> MQNSQDFSITELSLPKGGGAITGMGEALTPTGPDGMAALSLPLPISAGRGYAPAFTLNYNSGAGNSPFGLGWDCNVMTIRRRTHFGVPHYDETDTFLGPEGEVLVVADQPRDESTLQGINLGATFTVTGYRSRLESHFSRLEYWQPKTTGKTDFWLIYSPDGQVHLLGKSPQARISNPSQTTQTAQWLLEASVSSRGEQIYYQYRAEDDTGCEADEITHHLQATAQRYLHIVYYGNRTASETLPGLDGSAPSQADWLFYLVFDYGERSNNLKTPPAFSTTGSWLCRQDRFSRYEYGFEIRTRRLCRQVLMYHHLQALDSKITEHNGPTLVSRLILNYDESAIASTLVFVRRVGHEQDGNVVTLPPLELAYQDFSPRHHAHWQPMDVLANFNAIQRWQLVDLKGEGLPGLLYQDKGAWWYRSAQRLGEIGSDAVTWEKMQPLSVIPSLQSNASLVDINGDGQLDWVITGPGLRGYHSQRPDGSWTRFTPLNALPVEYTHPRAQLADLMGAGLSDLVLIGPKSVRLYANTRDGFAKGKDVVQSGDITLPVPGADPRKLVAFSDVLGSGQAHLVEVSATKVTCWPNLGRGRFGQPITLPGFSQPATEFNPAQVYLADLDGSGPTDLIYVHTNRLDIFLNKSGNGFAEPVTLRFPEGLRFDHTCQLQMADVQGLGVASLILSVPHMSPHHWRCDLTNMKPWLLNEMNNNMGVHHTLRYRSSSQFWLDEKAAALTTGQTPVCYLPFPIHTLWQTETEDEISGNKLVTTLRYARGAWDGREREFRGFGYVEQTDSHQLAQGNAPERTPPALTKNWYATGLPVIDNALSTEYWRDDQAFAGFSPRFTTWQDNKDVPLTPEDDNSRYWFNRALKGQLLRSELYGLDDSTNKHVPYTVTEFRSQVRRLQHTDSRYPVLWSSVVESRNYHYERIASDPQCSQNITLSSDRFGQPLKQ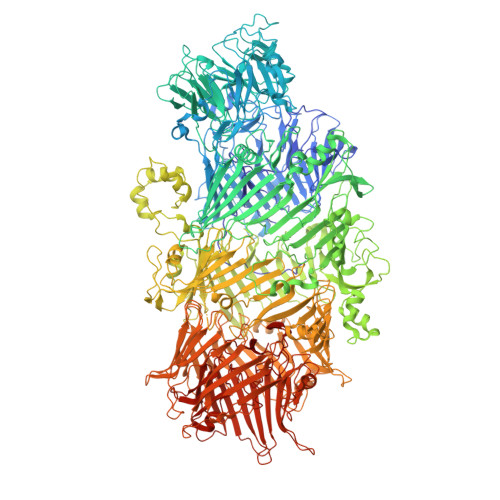LSVQYPRRQQPAINLYPDTLPDKLLANSYDDQQRQLRLTYQQSSWHHLTNNTVRVLGLPDSTRSDIFTYGAENVPAGGLNLELLSDKNSLIADDKPREYLGQQKTAYTDGQNTTPLQTPTRQALIAFTETTVFNQSTLSAFNGSIPSDKLSTTLEQAGYQQTNYLFPRTGEDKVWVAHHGYTDYGTAAQFWRPQKQSNTQLTGKITLIWDANYCVVVQTRDAAGLTTSAKYDWRFLTPVQLTDINDNQHLITLDALGRPITLRFWGTENGKMTGYSSPEKASFSPPSDVNAAIELKKPLPVAQCQVYAPESWMPVLSQKTFNRLAEQDWQKLYNARIITEDGRICTLAYRRWVQSQKAIPQLISLLNNGPRLPPHSLTLTTDRYDHDPEQQIRQQVVFSDGFGRLLQAAARHEAGMARQRNEDGSLIINVQHTENRWAVTGRTEYDNKGQPIRTYQPYFLNDWRYVSNDSARQEKEAYADTHVYDPIGREIKVITAKGWFRRTLFTPWFTVNEDENDTAAEVKKVKMPGSRPMKNIDPKLYQKTPTVSVYDNRGLIIRNIDFHRTTANGDPDTRITRHQYDIHGHLNQSIDPRLYEAKQTNNTIKPNFLWQYDLTGNPLCTESIDAGRTVTLNDIEGRPLLTVTATGVIQTRQYETSSLPGRLLSVAEQTPEEKTSRITERLIWAGNTEAEKDHNLAGQCVRHYDTAGVTRLESLSLTGTVLSQSSQLLIDTQEANWTGDNETVWQNMLADDIYTTLSTFDATGALLTQTDAKGNIQRLAYDVAGQLNGSWLTLKGQTEQVIIKSLTYSAAGQKLREEHGNDVITEYSYEPETQRLIGIKTRRPSDTKVLQDLRYEYDPVGNVISIRNDAEATRFWHNQKVMPENTYTYDSLYQLISATGREMANIGQQSHQFPSPALPSDNNTYTNYTRTYTYDRGGNLTKIQHSSPATQNNYTTNITVSNRSNRAVLSTLTEDPAQVDALFDAGGHQNTLISGQNLNWNTRGELQQVTLVKRDKGANDDREWYRYSGDGRRMLKINEQQASNNAQTQRVTYLPNLELRLTQNSTATTEDLQVITVGEAGRAQVRVLHWESGKPEDIDNNQLRYSYDNLIGSSQLELDSEGQIISEEEYYPYGGTALWAARNQTEASYKTIRYSGKERDATGLYYYGYRYYQPWIGRWLSSDPAGTIDGLNLYRMVRNNPVTLLDPDGL>CCGCCGGCGG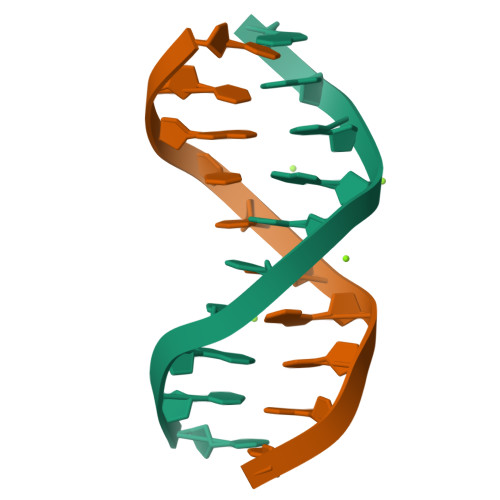[2x]>[2x]GPKFPRVKNWELGSITYDTLCAQSQQDGPCTPRRCLGSLVLPRKLQTRPSPGPPPAEQLLSQARDFINQYYSSIKRSGSQAHEERLQEVEAEVASTGTYHLRESELVFGAKQAWRNAPRCV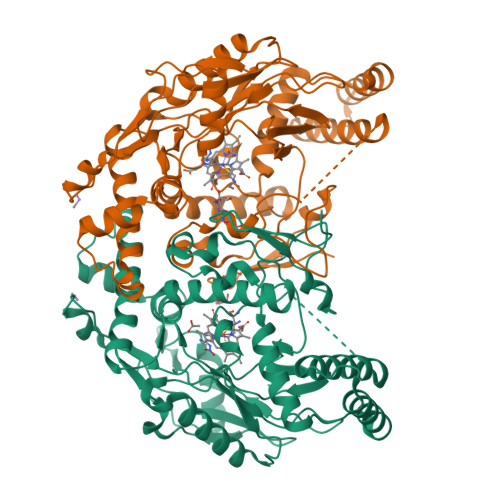GRIQWGKLQVFDARDCSSAQEMFTYICNHIKYATNRGNLRSAITVFPQRAPGRGDFRIWNSQLVRYAGYRQQDGSVRGDPANVEITELCIQHGWTPGNGRFDVLPLLLQAPDEAPELFVLPPELVLEVPLEHPTLEWFAALGLRWYALPAVSNMLLEIGGLEFSAAPFSGWYMSTEIGTRNLCDPHRYNILEDVAVCMDLDTRTTSSLWKDKAAVEINLAVLHSFQLAKVTIVDHHAATVSFMKHLDNEQKARGGCPADWAWIVPPISGSLTPVFHQEMVNYILSPAFRYQPDPWK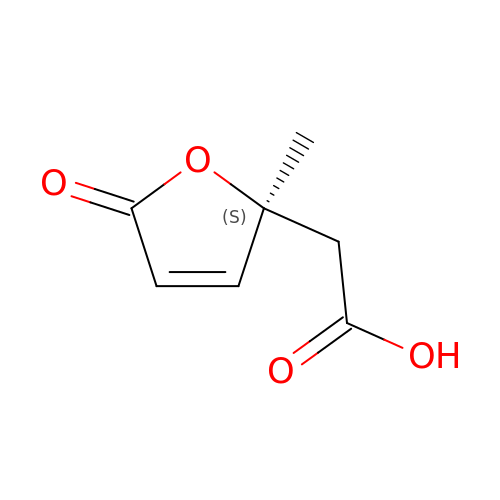[(2S)-2-methyl-5-oxo-2,5-dihydrofuran-2-yl]acetic acid | C7 H8 O4 | FIKLRROSHXQNFN-SSDOTTSWSA-N> MILDTD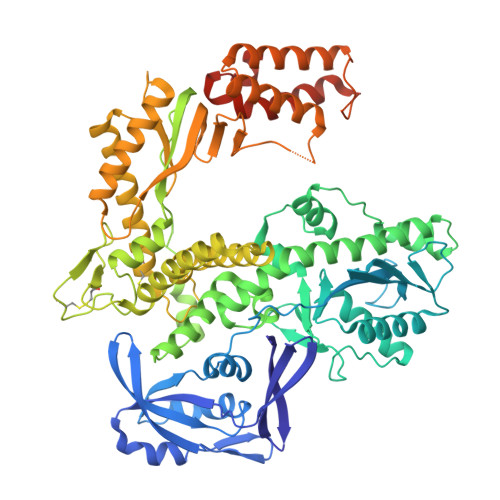YITEDGKPVIRIFKKENGEFKIDYDRNFEPYIYALLKDDSAIEDVKKITAERHGTTVRVVRAEKVKKKFLGRPIEVWKLYFTHPQDQPAIRDKIKEHPAVVDIYEYDIPFAKRYLIDKGLIPMEGDEELKMLAFAIATLYHEGEEFAEGPILMISYADEEGARVITWKNIDLPYVDVVSTEKEMIKRFLKVVKEKDPDVLITYNGDNFDFAYLKKRSEKLGVKFILGREGSEPKIQRMGDRFAVEVKGRIHFDLYPVIRRTINLPTYTLEAVYEAIFGQPKEKVYAEEIAQAWETGEGLERVARYSMEDAKVTYELGKEFFPMEAQLSRLVGQSLWDVSRSSTGNLVEWFLLRKAYERNELAPNKPDERELARRRESYAGGYVKEPERGLWENIVYLDFRSLYPSIIITHNVSPDTLNREGCEEYDVAPQVGHKFCKDFPGFIPSLLGDLLEERQKVKKKMKATIDPIEKKLLDYRQRLIKILANSFYGYYGYAKARWYCKECAESVTAWGRQYLETTIREIEEKFGFKVLYADTDGFFATIPGADAETVKKKAKEFLDYINAKLPGLLELEYEGFYKRGFFVTKKKYAVIDEEDKITTRGLEIVRRDWSEIAKETQARVLEAILKHGDVEEAVRIVKEVTEKLSKYEVPPEKLVIYKQITRDLKDYKATGPHVAVAKRLAARGIKIRPGTVISYIVLKGSGRIGDRAIPFDEFDPAKHKYDAEYYIENQVLPAVERILRAFGYRKEDLRYQKTRQVGLGAWLKPKT4-[[2-(4-oxidanylidenebutanoyl)hydrazinyl]methyl]benzoic 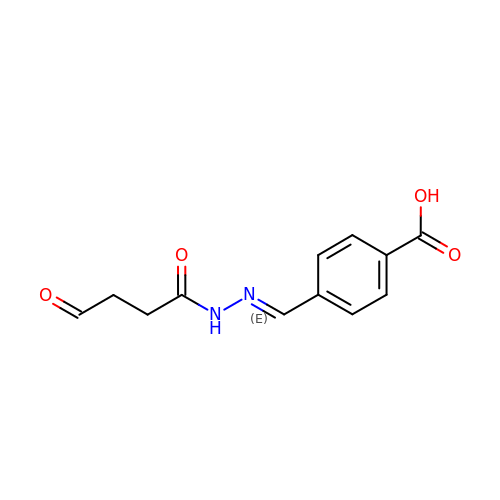acid | C12 H12 N2 O4 | YBTAMVPSZKNTLP-MDWZMJQESA-N> MGSSHHHHHHMDRYEIKGVDVASYQG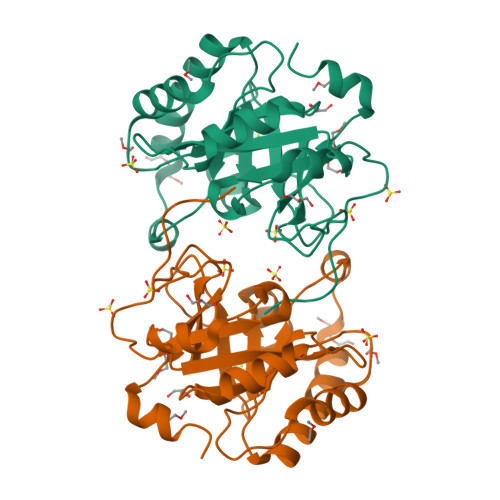DIDWRELEKQNMKFAFIKATEGSAFVDKYFSKNWTNANKTSMRVGAYHFFSFDSKGETQAEQFIRNVPKYKQALPPVIDVEFYANKKDNPPKREDVTKELSVMIEMLEKHYGKKVILYATQEAYDLYIKDAYPQCDIWIRSVLTKPSLSDERKWTFWQYTNRGKLSGYNGKEKYIDLNVFYGNEEEFENYGMKD>[2x]MSVLFISDLHLEAERPDITRAFLSFLDERARRAEALYILGDFFEAWIGDDGMDAFQRSIAQSLRQVADGGTRIYLMHGNRDFLIGKAFCREAGCTLLPDPSVIDLYGEPVLLMHGDSLCTRDEAYMRLRRWLRNPLTLWVLRHLPLATRHKLARKLRKESRAQTRMKAVDIIDVTPEEVPRVMRGHGVRTLIHGHTHRPAEHPLDIDGQPARRIVLGDWDRQGWALEIDANGHRQAPFPLLEHHHHHH

In the fourth step in this pathway, UDP-2,3-diacylglucosamine is hydrolyzed to 2,3-diacylglucosamine-1-phosphate (also called lipid X) and UMP. This step is catalyzed by the specific pyrophosphatase LpxH in 70% of gram-negative bacteria, including E. coli and Pseudomonas aeruginosa, and by LpxI in the remaining 30%345. LpxH shares sequence similarity with metallophosphoesterases and requires Mn2+ ions for phosphatase activity. PaLpxH consists of two domains: a catalytic domain homologous to metallophosphoesterases (MPEs) and a helical insertion domain (HI domain) inserted in the middle of the catalytic domain.

Proteins without Mn2+ ions were also successfully crystallized in two different space groups. A C2 form was obtained with no Mn2+ ions added during crystallization, and a P21 form was obtained by adding EDTA prior to crystallization. These crystals also contained two PaLpxH molecules in the asymmetric unit. No major changes were observed in the protein structures regardless of the presence of Mn2+ ions, suggesting that Mn2+ ions do not have a major effect on the protein structure.>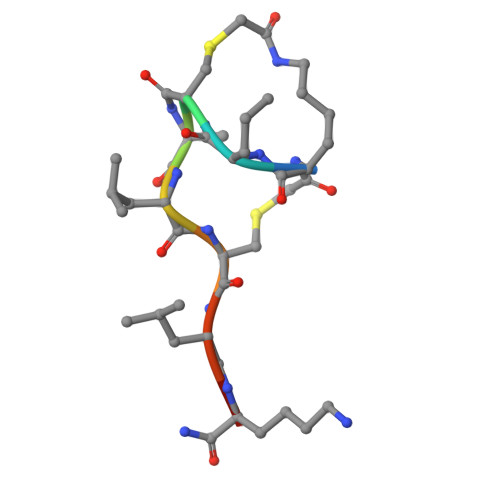 KKCKLCLKX3-(4-hydroxyphenyl)-6-methoxy-5,7-bis(oxidanyl)chromen-4-one | C16 H12 O6 | 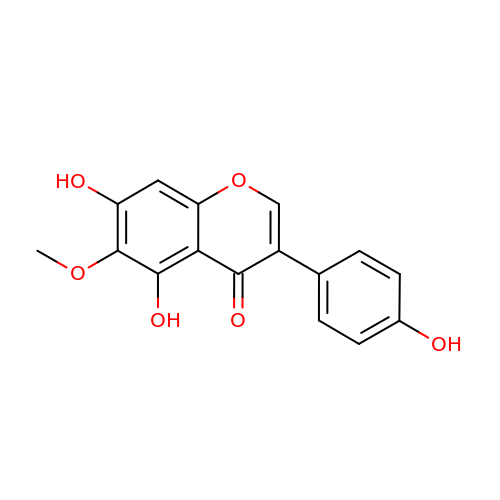OBBCRPUNCUPUOS-UHFFFAOYSA-N3-[2-(6-amino-4-methylpyridin-2-yl)ethyl]-5-{[2-(pyridin-2-yl)ethyl]amino}benzonitrile 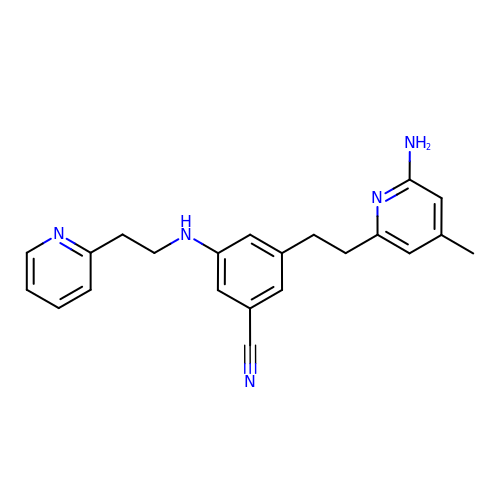| C22 H23 N5 | MPQMVSXQSZLJJB-UHFFFAOYSA-N3-FLUORO-4-HYDROXYBENZALDEHYDE O-(CYCLOHEXYLCARBONYL)OXIME | C14 H16 F N O3 | 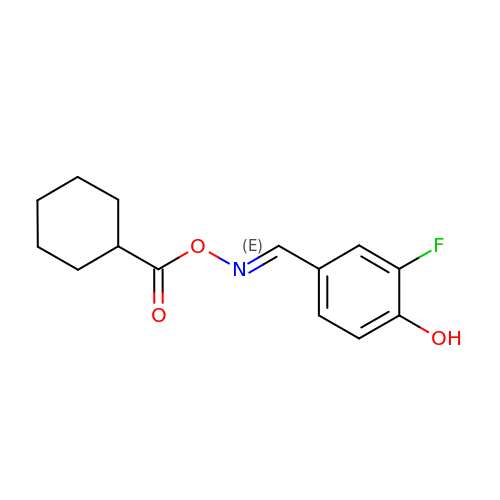NPVNUGQNVVMJJP-CXUHLZMHSA-N> MGSSHHHHHHSSGLVPRGSHMASDKPADSGSSEVKELTVYVDEGYKSYIEEVAKAYEKEAGVKVTLKTGDALGGLDKLSLDNQNGNVPDVMMAPYDRVGSLGSDGQLSEVKLSDGAKTDDTTKSLVTAANGKVYGAPAVIESLVMYYNKDLVKDAPKTFADLENLAKDSKYAF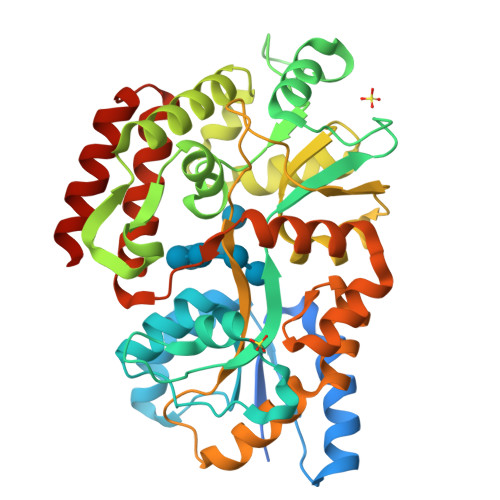AGEDGKTTAFLADWTNFYYTYGLLAGNGAYVFGQNGKDAKDIGLANDGSIVGINYAKSWYEKWPKGMQDTEGAGNLIQTQFQEGKTAAIIDGPWKAQAFKDAKVNYGVATIPTLPNGKEYAAFGGGKAWVIPQAVKNLEASQKFVDFLVATEQQKVLYDKTNEIPANTEARSYAEGKNDELTTAVIKQFKNTQPLPNISQMSAVWDPAKNMLFDAVSGQKDAKTAANDAVTLIKETLKQKFGE> AGLRHTFVVADATLPDCPLVYASEGFYAMTGYGPDEVLGHNCRFLQGEGTDPKEVQKIRDAIKKGEACSVRLLNYRKDGTPFWNLLTVTPIKTPDGRVSKFVGVQVDVTSKTEGKALA

Light–oxygen–voltage (LOV) domains are small photosensory flavoprotein modules that allow the conversion of external stimuli (sunlight) into intra­cellular signals responsible for various cell behaviors (e.g. phototropism and chloro­plast relocation). This ability relies on the light-induced formation of a covalent thio­ether adduct between a flavin chromophore and a reactive cysteine from the protein environment, which triggers a cascade of structural changes that result in the activation of a serine/threonine (Ser/Thr) kinase. For example, in the green algae Chlamydomonas reinhardtii (C. reinhardtii or Cr), phot allows the light-dependent regulation of several molecular processes (e.g. phototaxis, sexual differentiation, photoprotection) and control of gene expression. The C. reinhardtii phot protein consists of two successive photosensory protein modules, LOV1 and LOV2 domains, and a Ser/Thr kinase effector domain [Fig. 1(a)].

The recorded dark-state structure superimposed well with the deposited structure, showing a root-mean-square deviation (RMSD) of 0.15 Å (measured on the backbone Cα over 104 residues). However, compared with the previously published structure, we observed that the Arg74 side chain had rearranged (Chi3 57 to 4°) as it accommodated an altered rotamer of the flavin phospho­ribityl tail. The significant improvement in spatial resolution also allowed us to model Leu34, Val103, Ile73 and Cys32 residues surrounding the flavin in alternate conformations [Fig. S2(a)], revealing system equilibrium dynamics and several water molecules coordinating the phospho­ribityl tail and the phosphate group [Fig. S2(b)]. Overall, the electron density was of excellent quality and enabled us to observe variations in the positions of residue side chains (with an RMSD of 0.189 Å between the dark state at CT and RT). The reactive cysteine (Cys57) exhibited two alternate conformations, as observed at CT, but the variation of the 2Fo − Fc map contour at RT clearly indicated a change in the distribution of each conformation [Figs. 3(a) and 3(b), respectively]. We thus refined the occupancy of cysteine using Phenix for both temperatures. Conformation A, in which the Sγ atom of Cys57 is 3.5 Å from the C4a of FMN, was equally present at RT along with conformation B (i.e. 0.50 and 0.50 for A and B conformations, respectively), in which the Sγ atom of Cys57 is 4.4 Å from the C4a of FMN. However, at CT, conformation A is favored (with an occupancy of 0.70 compared with 0.30 for conformation B).>[4x]AQSLSFSFTKFDPNQEDLIFQGHATSTNNVLQVTKLDSAGNPVSSSAGRVLYSAPLRLWEDSAVLTSFDTIINFEISTPYTSRIADGLAFFIAPPDSVISYHGGFLGLFPNAN;>[4x]SNVVAVEFDTYLNPDYGDPNYIHIGIDVNSIRSK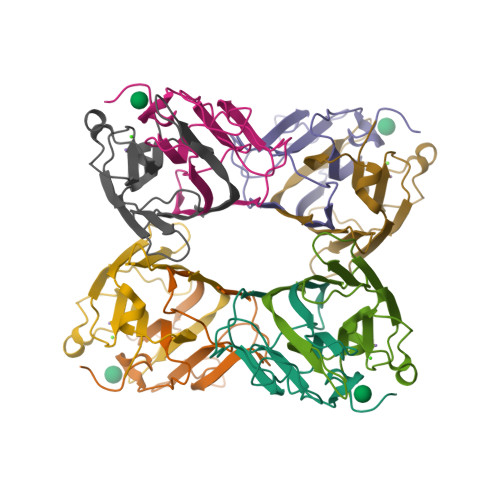VTAKWDWQNGKIATAHISYNSVSKRLSVTSYYAGSKPATLSYDIELHTVLPEWVRVGLSASTGQDKERNTVHSWSFTSSLWTNVAKKENENKYITRGVL>MGSSHHHHHSSGLVPRGSHMAVIPNFHLPMRSFEVKNRTSVDDIKSLRLITAIKTPYLPDGRFDLEAYDALVNMQIVDGAEGVIVGGTTGEGQLMSWDEHIMLIGHTVNCFGGSIKVIGNTGSNSTREA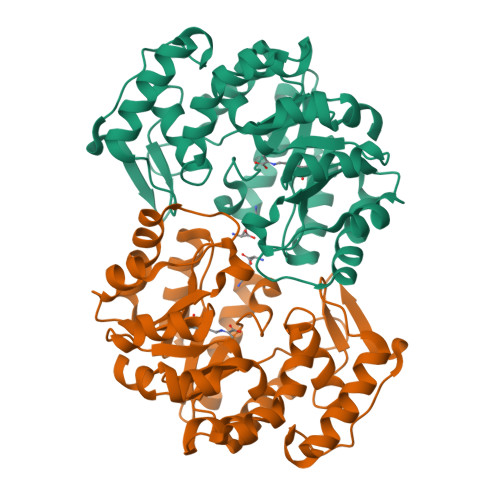IHATEQGFAVGMHAALHINPYYGKTSLEGLVSHFESVLPMGPTVIYNVPSRTGQDIPPGVIHTVAQSANLAGVKECVGNDRIKQYTDNRIVVWSGNDDQCHDAKWDYGATGVISVTSNLIPGLMRQLLFKGKNPSLNAKIMPLVNWLFEEPNPIGLNTALAQLGVVRPVFRLPYVPLPLAKRVEFVNIVKEIGRENFVGEKDVKVLDDDDFILVGRY[8x]>[6x]MNGKFADGPYSGILDSVLDAIGNTPMVRMKRLAKVYGLECDLLAKCEFMSAGGSVKDRIGKAMVEKAEREGRLKAGDTLIEPTSGNTGIGLALAAAVRGYRMIVTMPAKMSAEKSNIMKCLGAEIVRTPTEAAWNDENSHMGVAAKLQRELENAHILDQYNNTANPMVHYDVTAEEIITQCDGDIDMVVIGAGTGGTITGIGRKIKERCPKCKVVGVDPKGSILAVPDSLNDEKRLQSYEVEGIGYDFVPGVLDRKVVDEWVKVGDAESFTTARAIIRNEGLFVGGSSGANVWGALQAARQLKKGQKCVVLLPDSSRNYMSKFISDEWMAEHGFAPEDGAKVKEREKQFGGARIRDLLSETGATSDVPFVTARLSVEDVIKMMHETKVKEVIVTEDSEADGKTK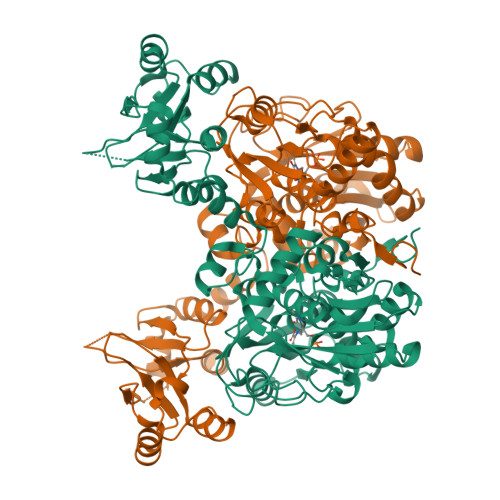LVGVLSEDHIAHSLQSGRCAMQSPVKDIAFKKLAKALPSAYLRDVAKALDFSPYVCVMDEKPSTKKQAGMGEHERAKISLRKAGNSRECPHFLGVITRIDLLHWLATKQK> MANKAVNDFILAMNYDKKKLLTHQGESIENRFIKEGNQLPDEFVVIERKKRSLSTNTSDISVTA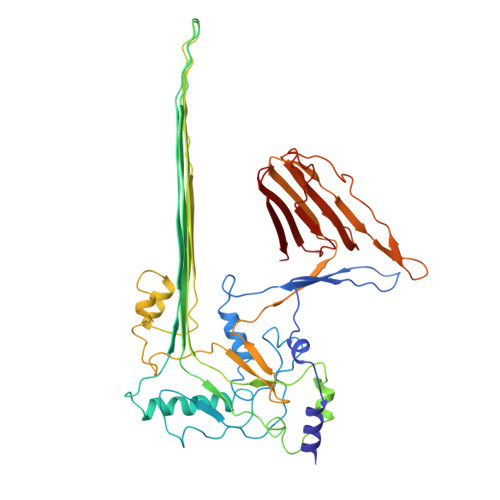TNDSRLYPGALLVVDETLLENNPTLLAVDRAPMTYSIDLPGLASSDSFLQVEDPSNSSVRGAVNDLLAKWHQDYGQVNNVPARMQYEKITAHSMEQLKVKFGSDFEKAANSLDIDFNAVHSGEKQIQIVNFKQIYYTVSVDAVKNPGDVFQDTVTVEDLKQRGISAERPLVYISSVAYGRQVYLKLETTSKSDEVQAAFEAAILGVKVAPQTQWKQILDNTEVKAVILGGDPSSGARVVTGKVDMVEDLIQEGSRFTADHPGLPISYTTSFLRDNVVATFQNSTDYVETKVTAYRNGDLLLDHSGAYVAQYYITWDELSYDHQGKEVLTPKAWDRNGQDLTAHFTTSIPLKGNVRNLSVKIRECTGLAWEWWRTVYEKTDLPLVRKRTISIWGTTLYPQVEDKVEND> MSLGAKPFGEKKFIEIK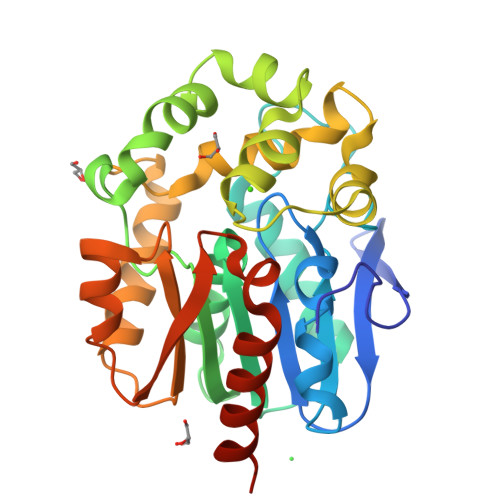GRRMAYIDEGTGDPILFQHGNPTSSYLWRNIMPHCAGLGRLIACDLIGMGDSDKLDPSGPERYTYAEHRDYLDALWEALDLGDRVVLVVHDWGSVLGFDWARRHRERVQGIAYMEAVTMPLEWADFPEQDRDLFQAFRSQAGEELVLQDNVFVEQVLPGLILRPLSEAEMAAYREPFLAAGEARRPTLSWPRQIPIAGTPADVVAIARDYAGWLSESPIPKLFINAEPGHLTTGRIRDFCRTWPNQTEITVAGAHFIQEDSPDEIGAAIAAFVRRLRPAHHHHHH> GPGSMADSCIFCKIAQKQIPSTIVYEDDEIFAFKDINPIAPIHILVIPKQHIASLNEITEENEAFIGKVLYKVSLIGKKECPEGYRVVNNIGED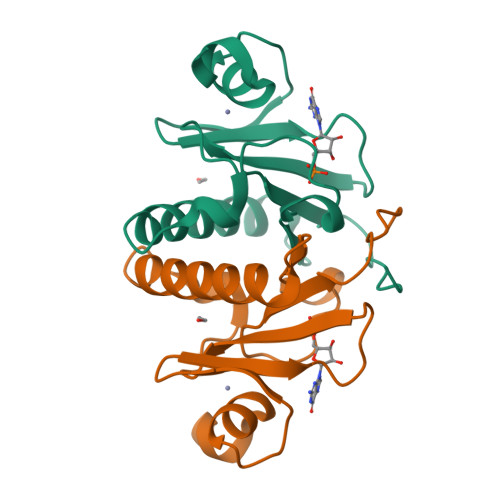AGQTVKHIHFHILGGKKLAWDKL> MSDIRHSLLRRDALSAAKEVLYHLDIYFSSQLQSAPLPIVDKGPVELLEEFVFQVPKERSAQPKRLNSLQELQLLEIMCNYFQEQTKDSVRQIIFSSLFSPQGNKADDSRMSLLGKLVSMAVAVCRIPVLEC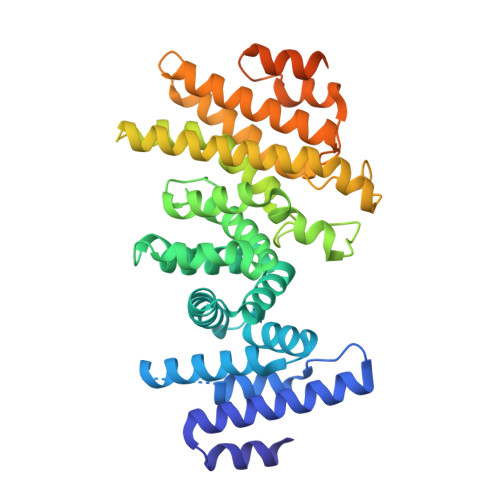AASWLQRTPVVYCVRLAKALVDDYCCLVPGSIQTLKQIFSASPRFCCQFITSVTALYDLSSDDLIPPMDLLEMIVTWIFEDPRLILITFLNTPIAANLPIGFLELTPLVGLIRWCVKAPLAYKRKKKPPLSNGHVSNKVTKDPGVGMDRDSHLLYSKLHLSVLQVLMTLQLHLTEKNLYGRLGLILFDHMVPLVEEINRLADELNPLNASQEIELSLDRLAQALQVAMASGALLCTRDDLRTLCSRLPHNNLLQLVISGPVQQSPHAALPPGFYPHIHTPPLGYGAVPAHPAAHPALPTHPGHTFISGVTFPFRPIR> LRWSRLLRGRPPPVMGHAKRMRFAGVDDNPSVTHKPWDTSEPLMADYGWERGKLPKFRARSPFHRQQI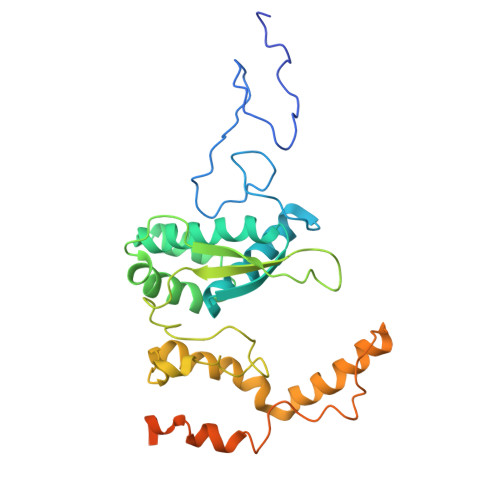ARRMVTELIRKDYVIVGGARAPALRILADHVVELAKAGDTDSRQQLAYFLHDPLMVDKAFDEYPRRFRDMNAKYAMMTRLKGRRRSDNVAMYFVEYKNRDMSDNHKGEDYTAGPERFFLPPRIIETEKGIQRPPHMQMAFDRWASKFKTEEFHHWWRLRHAKLRYWGVRNVPHPSDVDPLWTEKEEEEWHNEMLANTSDFEDFDLDDDSYEAAGEGGSQGGSSSLSGIGPEPQKKY>[6x]MRIGYGEDSHRLEEGRPLYLCGLLIPSPVGALAHSDGDAALHALTDALLSAYGLGDIGLLFPDTDPRWRGERSEVFLREALRLVEARGAKLLQ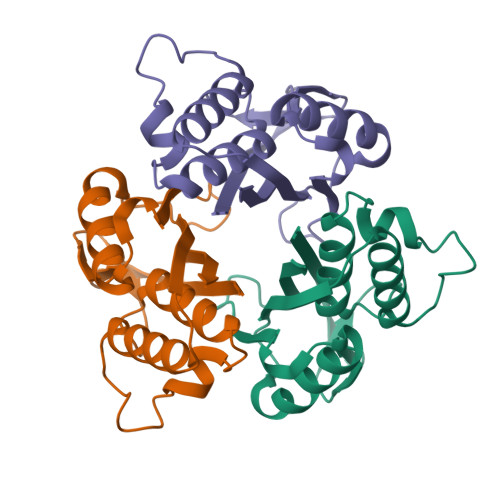ASLVLTLDRPKLGPHRKALVDSLSRLLRLPQDRIGLTFKTSEGLAPSHVQARAVVLLDG Many folds, spanning all levels of complexity (fibrous, solenoid, toroid, and globular), clearly originated in this way. β-Propellers offer an attractive model system to study this process. They are toroids formed by sequential supersecondary structure units of typically 40–50 residues, each consisting of four anti-parallel β-strands. The units are arranged radially, with their strands perpendicular to the plane of the toroid, and have a right-handed twist, hence the name ‘propeller’ for the fold and ‘blades’ for the repetitive units. Since none of our single-bladed PkwA constructs were folded, we turned our attention to another highly symmetric β-propeller of the WD40 family, found in the C-terminal part of Npun_R6612 from the multicellular cyanobacterium Nostoc punctiforme PCC 73102 and referred to henceforth as WRAP (WD40-family Recently Amplified Propeller; ACC84870.1). WRAP, which we identified during a systematic bioinformatic survey of β-propellers, was particularly interesting in that its 14 blades are practically identical, having acquired only 10 point mutations over 563 residues (6 of these being Trp → Arg mutations at the same position of blades 1, 3, 6, 10, 12, and 13), as a result of 13 non-synonymous substitutions at the DNA level.

For the 3-bladed construct, SLS data indicated a trimer, as also suggested by our crosslinking data. This result is in contrast to the aforementioned 3-bladed PkwA construct which formed dimers, pointing to a certain versatility in the way different fragments with the same repeat number can assemble. As we anticipated from their oligomeric states, the 2-bladed and 4-bladed fragments formed 8-bladed propellers and the 3-bladed fragment a 9-bladed propeller. Instead, the packing of the blades within each fragment preserves the geometry of the 7-bladed parent, and the tension due to the mismatch between the number of blades in the assembly versus that in the parent accumulates at the interface between the fragments. In the 9-bladed propeller, the symmetry mismatch is absorbed to equal extent at three interfaces, leading to a slightly triangular shape.

>GAMGSSSVWGVAFSPDGQTIASASDDKTVKLWNRNGQLLQTLTGHSSSVWGVAFSPDGQTIASASDDKTVKLWNRNGQLLQTLTGHSSSVWGVAFSPDGQTIASASDDKTVKLWNRNGQLLQTLTGH[6x]In this publication, we present the three-dimensional structure of the tandem PX-PH domains of the yeast protein Bem3.

In this study, we have determined the X-ray crystallographic structure of the interesting tandem PX-PH domain module of Bem3 to a resolution of 2.2 Å, showing that the putative membrane-binding regions of both domains are oriented in the same direction and thus might act synergistically in membrane recognition and binding. The crystal structure of the tandem PX-PH domains shows the well characterized folds of both protein domains. The model contains amino acids 502–629 belonging to the PX domain and 636–737 of the PH domain, but the linker region (amino acids 630–635) between the domains as well as the loops between β1PH and β2PH (amino acids 647–651) and β6PH and β7PH (amino acids 709–715) within the PH domain were flexible and could not be resolved. Even though six amino acids are missing between the two domains, the presented structural assembly within the asymmetric unit represents the only possible arrangement, and a different connectivity between the PX and PH domains is excluded because the positions of the respective C- and N-termini are too remote. Strikingly, the PX domain of Bem3 contains basic residues (for example Lys551 and Arg592/Lys593) at similar positions compared with other PX domains, which have previously been termed basic motifs I and II, respectively, and have been shown to be involved in PIP binding. Specific point mutations introduced at this position in Slm1 and the PH domain of EFA6 resulted in mislocalization of the respective proteins, further signifying the role of this arginine in ligand binding. In line with these findings, an analysis involving the mutation of basic residues within the β1PH–β2PH loop of yeast Bem3 (R644S, R645S and K647D) showed that this abolished binding of the PH domain to PIP2, rendering the protein incapable of correctly localizing to the polar site at the cell membrane. In contrast to these mutations within the PH domain, a quadruple mutant (Y524W, R578S, L580S and F581M; Mukherjee et al., 2013) involving amino acids within the so-called ‘membrane-interaction loop’ of the PX domain exhibits wild-type localization of Bem3. Although the critical residues Lys551 and Arg592 of basic motifs I and II of the Bem3 PX domain are conserved in the majority of PX domains, their role in the direct binding of PIPs has yet to be elucidated. The structure shows that the putative lipid-binding domains adopt a relative orientation that enables them to simultaneously bind to a membrane.

> GHMKSDIPLFVQPEDFGTIQIEVLSTLYRDNEDDLSILIAIIDRKSGKEMFKFSKSIHKVRELDVYMKSHVPDLPLPTLPDRQLFQTLSPTKVDTRKNILNQYYTSIFSVPEFPKNVGLKIAQFISTDTVMTPPMMDDNVKDGSLLLRRPKTLTGNSTWRVRYGILRDDVLQLFDKNQLTETIKLRQSSIELIPNLPEDRFGTRNGFLITEHKKSGLSTSTKYYICTETSKERELWLSAFSDYIDPSQSLSLSSSRNANDTDSASHLSA> MIHCLRNIRTVSALQSKISYNLGGGNKRKKTSGDLDNYDVLFVGANLGGICSNHFDKDTHGKYKCFVSFDQPINQIYSVRIPYEQQRVRKSEYIHFSKKSINQFTPSEMLAVKEILPEQNAVVLSSGRRIGYNQLVLATGLKHDFSQIKGFYEALEHPEHPVYANRDPETWRSAQHKYSKYISNFKSGDGYFCIPEYPYAGEVECFNFFVSDEVWKWAQHHGALSPKHTFTIVNANEKFVHYCDSADAFIKERLEKRGIRVEYNTKLLEVHQDGQKATFINTKTGEKSVRDYNNLYSIVPSKRQEFLDKAGLTNGNGLLNVDHQTLQHKKYKNIFGLGDAADLPTTKTFWAGWYQIAVVRNNVKRNLQGQTLNAHYDGFSKVPLFTGHQTLTYVAHSYGGVGNWQHLKHNNGGILAWMRYRSWAKGMAKKFQDFYNGARLGPPYHKVLKSFPELPGSPESQQSSGISKYFPTKTENKAAH

The F-type ATP synthase (F1Fo-ATP synthase) is responsible for generating most of the cellular adenosine triphosphate (ATP) from adenosine diphosphate (ADP) and inorganic phosphate through rotary catalysis. In eukaryotes, ATP synthases are found in the inner mitochondrial membrane. The type III ATP synthase was detected in ciliates where it induces tubulation of the cristae membranes. In this study, we present the cryo-EM structures of the type III ATP synthase dimer and tetramer with associated lipids from the model organism Tetrahymena thermophila in complex with the natural inhibitor IF1.

Using masked refinements, the resolution of different regions reached 2.5–3.1 Å, allowing de novo modelling. The Fo-wing clamps around the c-ring, and is formed by a 55-kDa subunit ATPTT1. Its tertiary fold superposes well with that of human mitochondrial sulfide:quinone oxidoreductase, which uses flavin adenine dinucleotide (FAD) for its activity. However, in ATPTT1 the binding pocket formed by two Rossmann folds contains the co-factor nicotinamide adenine dinucleotide (NAD). The nicotinamide group of the NAD is in close proximity to Cys205, which could potentially be the active site of ATPTT1. The human sulfide:quinone oxidoreductase is an integral membrane protein, and ATPTT1 locates closely to the matrix leaflet of the crista membrane with several adjacent lipid-like density features resolved in the cryo-EM density map. Thus, ATPTT1 is positioned to encounter membrane-embedded electron-acceptors, such as CoQ, in a similar fashion as the human enzyme.>[2x]RLACKEDYRYAISSTNEIGLLGAGGLTTTWKEYSHDLQLNDGTVKAICVAGSFKITALNVVSRRYLASLHKGALLTSVTFELLFDGTNPSTEEMGDDFGFGLCPFDTSPVVKGKYNTTLLNGSAFYLVCPIGWTGVIECTAVSPTTLRTEVVKTFRREKPFPHRMDCVTTTVE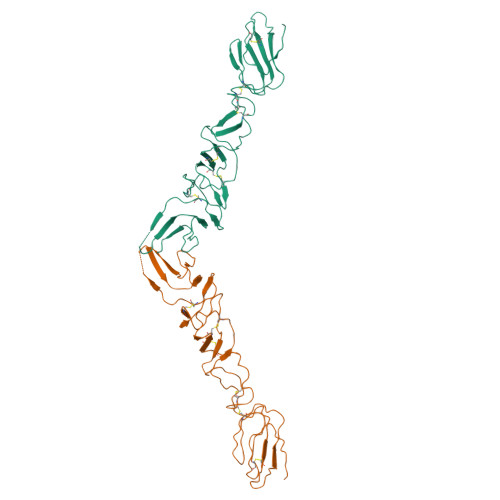NEDLFYCKLGGNWTCVKGEPVVYTGGQVKQCKWCGFDFNEPDGLPHYPIGKCILANETGYRIVDSTDCNRDGVVISAKGSHECLIGNTTVKVHASDERLGPMPCRPKEIVSSAGPVRKTSCTFNYAKTLKNKYYEPRDSYFQQYMLKGEYQYWFDLDVTDRHSGYFAEF As the first reported host of “non-pathogenic-derived” pili, Lactobacillus rhamnosus GG is a gut-adapted commensal lactic acid bacterium (LAB) and one of many clinically investigated probiotic strains for human use in the prevention and treatment of certain gastric ailments. As with other Gram-positive bacteria, sortase-dependent piliation in L. rhamnosus GG (called SpaCBA) is assembled from the ~30 kDa SpaA (backbone), ~20 kDa SpaB (basal), and ~90 kDa SpaC (tip-located) pilins. Two immunoglobulin (Ig)-like subdomains comprise GG-SpaA, each having the conserved residues of a canonical E-box motif and internal isopeptide bonds formed between either lysine and asparagine or lysine and aspartate residues. Our findings show that the GG-SpaA structure has certain features in common with other pathogen-derived pilin-proteins, such as the Ig-like CnaB-type folds and the presence of internal isopeptide bonds6940.

Crystals of full-length GG-SpaA protein belonging to the monoclinic C2 space group diffracted up to 1.9 Å resolution at a synchrotron source (BM14, ESRF). Crystals for full-length GG-SpaA contain three molecules in the asymmetric unit, where the head of one molecule faces the tail of another. Each GG-SpaA molecule is made up of two Ig-like domains connected by a short linker with an interface area of 641 Å2. The two domains are bent by a hinge angle31 (i.e., the angle between the principal ellipsoid axes of the domains) of 152°, in which the N- and C-terminal domains (N-domain and C-domain) consist of residues 39–175 and 176–302, respectively. The electron density map clearly shows continuous density for two intra-domain isopeptide bonds, one for each domain. Formation of the isopeptide bond (K-N) in the N-domain occurs between Lys47 at the end of β-strand A and Asn172 at the end β-strand G, which corresponds to the pilin motif found near the domain interface. On the other hand, isopeptide bond formation in the C-domain is between Lys184 from β-strand A and Asp295 from β-strand G, and involves a proximal catalytic Glu269 in a hydrophobic pocket made by Tyr276, Phe198, Ile293, Phe182, Phe245, Phe253, Ala196, and Leu193. Intriguingly, the three molecules present in the asymmetric unit of the GG-SpaA crystal are seen to generate what resembles a pilus-like fiber, and where the corresponding pilin molecules are in a “head-to-tail” arrangement that may reflect its native biological state. Along the axis of the pilus structure, each of the GG-SpaA molecules shows a rotation angle of ~120° and translation of ~78 Å. The inter-domain hinge angle (152°) in each GG-SpaA molecule and the head-to-tail positioning of adjoining molecules allow for the formation of an elongated spiral staircase-like arrangement that could then offer both flexibility and rigidity to SpaCBA pilus structure.

>MGRDPNSTNDTTTQNVVLTKYGFDKDVTAIDRATDQIWTGDGAKPLQGVDFTIYNVTANYWASPKDYKGSFDSAPVAATGTTNDKGQLTQALPIQSKDASGKTRAAVYLFHETNPRAGYNTSADFWLTLPAKAAADGNVYVYPKNVQKTTYERTFVKKDAETKEVLEGAGFKISNSDGKFLKLTDKDGQSVSIGEGFIDVLANNYRLTWVAESDATVFTSDKSGKFGLNGFADNTTTYTAVETNVPDGYDAAANTDFKADNSSSDILDAPSGILPLEHHHHHH[3x]> MKLDIKKTFSNRSDRVKGIDFHPTEPWVLTTLYSGRV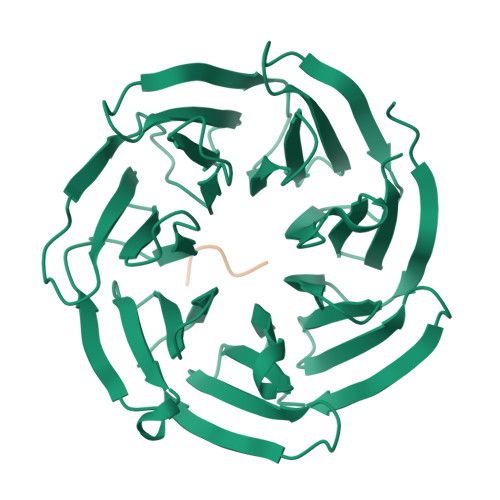EIWNYETQVEVRSIQVTETPVRAGKFIARKNWIIVGSDDFRIRVFNYNTGEKVVDFEAHPDYIRSIAVHPTKPYVLSGSDDLTVKLWNWENNWALEQTFEGHEHFVMCVAFNPKDPSTFASGCLDRTVKVWSLGQSTPNFTLTTGQERGVNYVDYYPLPDKPYMITASDDLTIKIWDYQTKSCVATLEGHMSNVSFAVFHPTLPIIISGSEDGTLKIWNSSTYKVEKTLNVGLERSWCIATHPTGRKNYIASGFDNGFTVLSLG;> KTKLL> ESKVVVPAQGKKITLQNGKLNVPENPIIPYIEGDGIGVDVTPAMLKVVDAAVEKAYKGERKISWMEIYTGEKSTQVYGQDVWLPAETLDLIREYRVAIKGPLTTPVGGGIRSLNVALRQELDLYI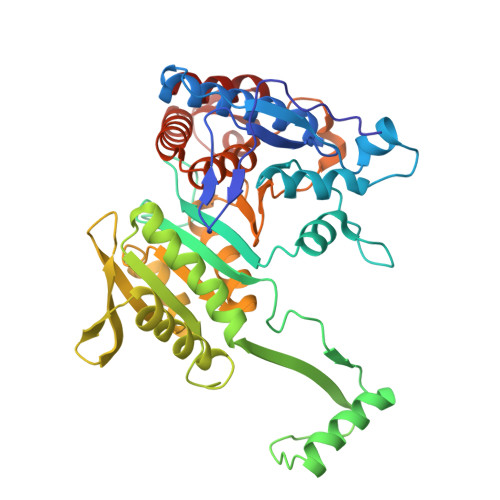CLRPVRYYQGTPSPVKHPELTDMVIFRENSEDIYAGIEWKADSADAEKVIKFLREEMGVKKIRFPEHCGIGIKPCSEEGTKRLVRAAIEYAIANDRDSVTLVHKGNIMKFTEGAFKDWGYQLAREEFGGELIDGGPWLKVKNPNTGKEIVIKDVIADAFLQQILLRPAEYDVIACMNLNGDYISDALAAQVGGIGIAPGANIGDECALFEATHGTAPKYAGQDKVNPGSIILSAEMMLRHMGWTEAADLIVKGMEGAINAKTVTYDFERLMDGAKLLKCSEFGDAIIENM>MAAAAVSGALGRAGWRLLQLRCLPVARCRQALVPRAFHASAVGLRSSDEQKQQPPNSFSQQHSETQGAEKPDPESSHSPPRYTDQGGEEEEDYESEEQLQHRILTAALEFVPAHGWTAEAIAEGAQSLGLSSAAASMFGKDGSELILHFVTQCNTRLTRVLEEEQKLV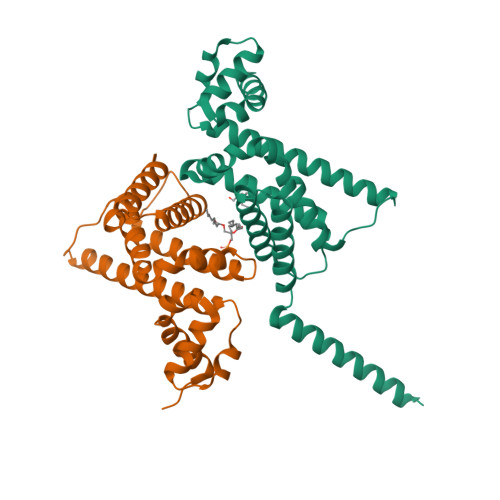QLGQAEKRKTDQFLRDAVETRLRMLIPYIEHWPRALSILMLPHNIPSSLSLLTSMVDDMWHYAGDQSTDFNWYTRRAMLAAIYNTTELVMMQDSSPDFEDTWRFLENRVNDAMNMGHTAKQVKSTGEALVQGLMGAAVTLKNLTGLNQRR[2x]>GHMLRGLRIIAENKIGVLRDLTTIIAEEGGNITFAQTFLIKHGEHEGKALIYFEIEGGDFEKILERVKTFDYIIEIEEEESFERVFGKRVIILGGGALVSQVAIGAISEADRHNLRGERISVDTMPVVGEEEIAEAVKAVSRLHRAEVLVLAGGIMGGKITEEVKKLRKSGIRVISLSMFGSVPDVADVVISDPVMAGTLAVMHISEKAKFDLDRVKGR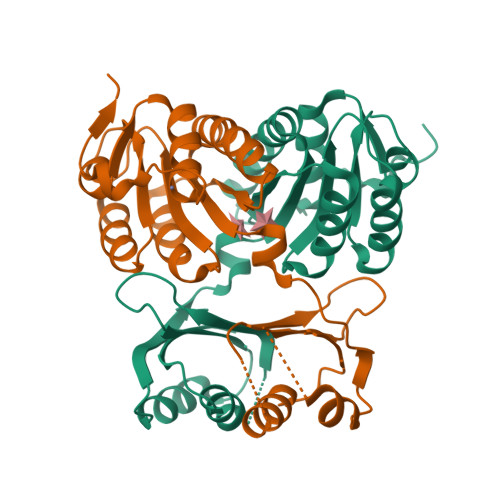RIGK[3x]>[2x]HHHHHHSSGLVPRGSHMFRSSLTHLQAASRVFIVGGHITPFVGKGSPLFIDKKHPDFGKKKNMTLEEILATTVQGTMEHSGLSGREGIVDQVVVGNFLGELFSSQGHLGPAAIGSLTYGQAGSKNPLMYKPAMRVEGAAASGGLAVISAMNALKSGSADITLAVGVEVQTTASARVGGDYLARAADYQRQRQLDDFTFPCLFAKRMKYIAEHNHFTMEDTARVAAKAYANGNKNPLAHMHTRKLT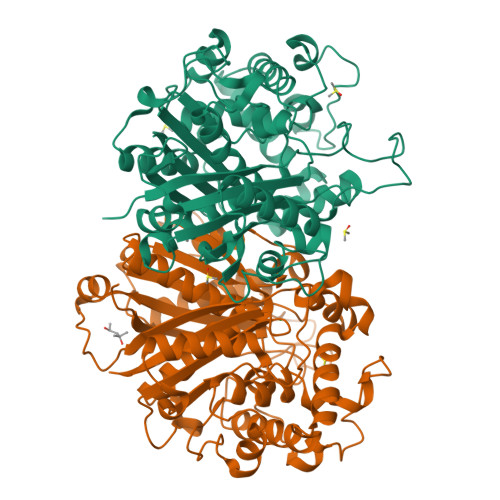FEQCNGEDPSNVKFLGNETYKEYLRMTDCSQVSDGGAGVVLANEEGLRKMGLSPNDSRLVEIKSIACAVSNLYEDPDDACCMFTSRQAAQKALSMANIKPSDLNVAEVHDCFTIAEMLMYEALGIAEYGHAKDLIRNGDTTLEGRIPVNTGGGLLSFGHPVGATGIKQIMEVYRQMKGQCEAYQMKKIPALGATLNMGGDDKTAVSAVLQNI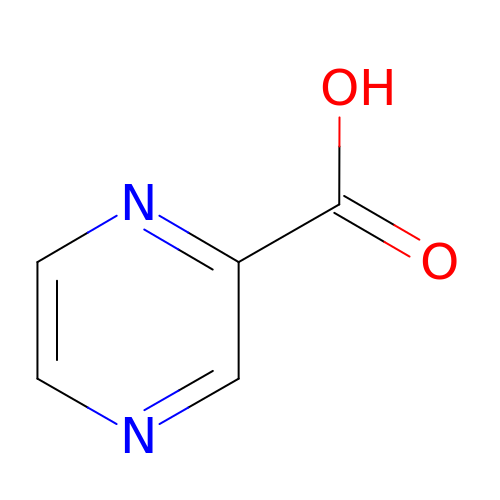PYRAZINE-2-CARBOXYLIC ACID | C5 H4 N2 O2 | NIPZZXUFJPQHNH-UHFFFAOYSA-N>MSVTVKRIIDNTVIVPKLPANEDPVEYPADYFRKSKEIPLYINTTKSLSDLRGYVYQGLKSGNVSIIHVNSYLYGALKDIRGKLDKDWSSFGINIGKAGDTIGIFDLVSLKALDGVLPDGVSDASRTSADDKWLPLYLLGLYRVGRTQMPEYRKKLMDGLTNQCKMINEQFEPLVPEGRDIFDVWGNDSNYTKIVAAVDMFFHMFKKHECASFRYGTIVSRFKDCAALATFGHLCKITGMSTEDVTTWILNREVADEMVQMMLPGQEIDKADSYMPYLIDFGLSSKSPYSSVKNPAFHFWGQLTALLLRSTRARNARQPDDIEYTSLTTAGLLYAYAVGSSADLAQQFCVGDNKYTPDDSTGGLTTNAPPQGRDVVEWLGWFEDQNRKPTPDMMQYAKRAVMSLQGLREKTIGKYAKSEFDK[3x];>[3x]MSSLKKILGLKGKGKKSKKLGIAPPPYEEDTSMEYAPSAPIDKSYFGVDEMDTYDPNQLRYEKFFFTVKMTVRSNRPFRTYSDVAAAVSHWDHMYIGMAGKRPFYKILAFLGSSNLKATPAVLADQGQPEYHAHCEGRAYLPHRMGKTPPMLNVPEHFRRPFNIGLYKGTIELTMTIYDDESLEAAPMIW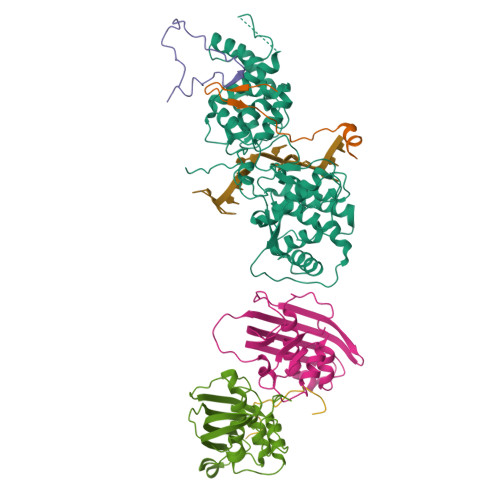DHFNSSKFSDFREKALMFGLIVEKKASGAWVLDSISHFK> EFLADSSAHLDLRNFYQLRDYRQHDAPQSQAGNWSQGFVLRLQSGFTGGPLGFGLDATGLLGVKLDSGRGRSNDGTLPFGANSKEPVDDYSHLGLTAKLRYSQTQLQVGILMPQLPVAFRDDVRLLPQTFDGALLTSSEIEGLTLTAGQLWKSRTRESAGSDDMYIMGRDKAHASDEFNLAGATYAFTPRLSASYYYGQLKDIYRQHYLGLLHTLPLGEGLSLRSDLRYFDSGEDGAAISGPVDNRNLNAMLTLRAGAHAFGIGVQKMIGNDAFPVLNGYTTPYVANLMAYQTFTRPQEKSWQLRYDYDFAGLGLPGLNLMTRYVQGRDIDRGAGRADDSEWERNTDLSYVIQSGPLKSV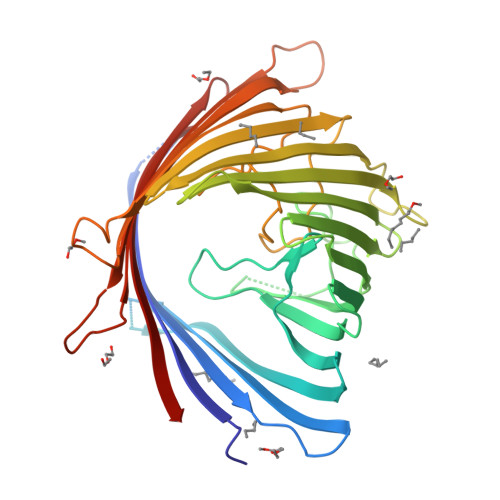ALKWRNITYRSRYGADLDENRFIVNYTLKLW> SGISLDN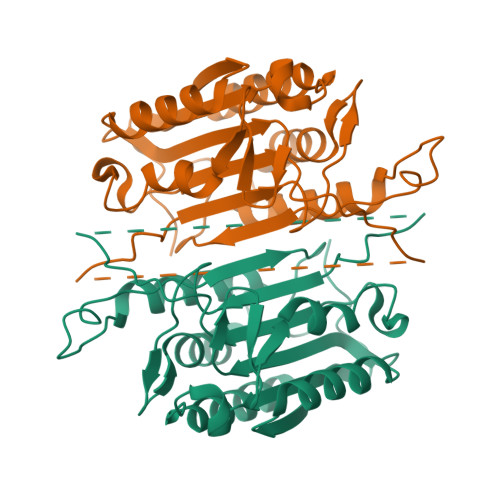SYKMDYPEMGLCIIINNKNFHKSTGMTSRSGTDVDAANLRETFRNLKYEVRNKNDLTREEIVELMRDVSKEDHSKRSSFVCVLLSHGEEGIIFGTNGPVDLKKITNFFRGDRCRSLTGKPKLFIIQACRGTELDCGIETDSGVDDDMACHKIPVDADFLYAYSTAPGYYSWRNSKDGSWFIQSLCAMLKQYADKLEFMHILTRVNRKVATEFESFSFDATFHAKKQIPCIVSMLTKELYFYHLEHHHHHH>MSNLLTVHQNLPALPVDATSDEVRKNLMDMFRDRQAFSEHTWKMLLSVCRSWAAWCKLNNRKWFPAEPEDVRDYLLYLQARGLAVKTIQQHLGQLNMLHRRSGLPRPSDSNAVSLVMRRIRKENVDAGERAKQALAFERTDFDQVRSLMENSDRCQDIRNLAFLGIAYNTLLRIAEIARIRVKDISRTDGGRMLIHIGRTATLVSTAGVEKALSLGVTKLVERWISVSGVADDPNNYLFCRVRKNGVAAPSATSQLSTRALEGIFEATHRLIYGAKDDSGQRYLAWSGHSARVGAARDMARAGVSIPEIMQAGGWTNVNIVMNYIRNLDS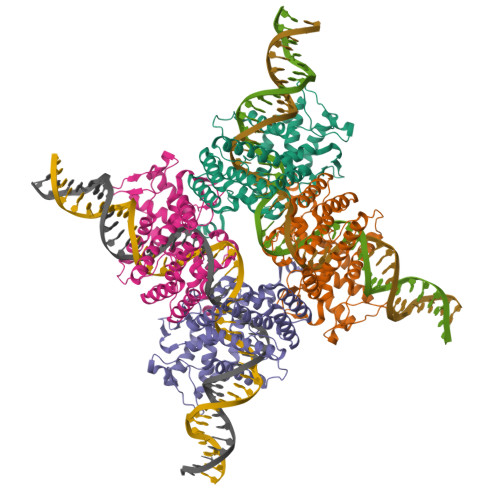ETGAMVRLLEDGD[4x]> MLMDEYEENKDMCPICKTDRYLSPDVKFLVNPECYHRICESCVDRIFSLGPAQCPYKGCDKIL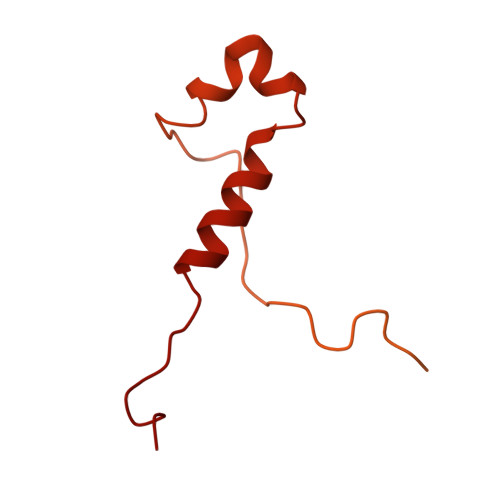RKNKFKTQIFDDVEVEKEVDIRKRVFNVFNKTIDDFNGDLVEYNKYLEEVEDIIYKLDHGIDVAKTEEKLRTYEELNKQLIMNNLERSRTEIESFEQRQKFEKEMKLKKRLLERQIEEEERMNKEWTKKEIVNRLSTTTQDINETIEGVKNTVKLKKSSARRKLEELNRVLKNNPYFNSNVNVQNSRLKDAVPFTPFNGDREAHPPFTLKGSVYNDPFIKDLEHRKEFIASGFNTNYAYERVLTEAFMGLGCVISEEL> PISPIETVPVKLKPGMDGPKVKQWPLTEEKIKALVEICTEMEKEGKISKIGPENPYNTPVFAIKKKDSTKWRKLVDFRELNKRTQDFWEVQLGIPHPAGLKKKKSVTVLDVGDAYFSV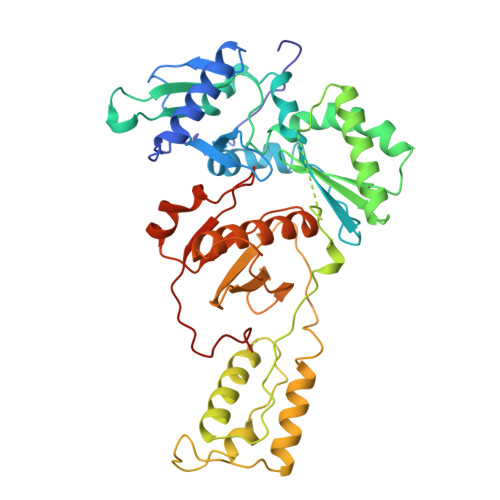PLDEDFRKYTAFTIPSINNETPGIRYQYNVLPQGWKGSPAIFQSSMTKILEPFRKQNPDIVIYQYMDDLYVGSDLEIGQHRTKIEELRQHLLRWGLTTPDKKHQKEPPFLWMGYELHPDKWTVQPIVLPEKDSWTVNDIQKLVGKLNWASQIYPGIKVRQLCKLLRGTKALTEVIPLTEEAELELAENREILKEPVHGVYYDPSKDLIAEIQKQGQGQWTYQIYQEPFKNLKTGKYARMRGAHTNDVKQLTEAVQKITTESIVIWGKTPKFKLPIQKETWETWWTEYWQATWIPEWEFVNTPPLVKLWYQLEKEPIVGAETF> MGMIVFVRFNSSYGFPVEV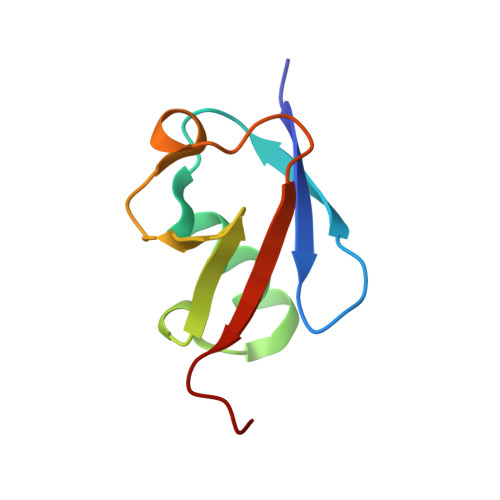DSDTSILQLKEVVAKRQGVPADQLRVIFAGKELPNHLTVQNCDLEQQSIVHIVQRPRRR>DPIHYDKITEEINKAIDDAIAAIEQSETIDPMKVPDHADKFERHVGILDFKGELAMRNIEARGLKQMKRQGDANVKGEEGIVKAHLLIGVHDDIVSMEYDLAYKLGDLHPTTHVISDIQDFVVALSLEIPDEGNITMTSFEVRQFANVVNHIGGLSILDPIFGVLSDVLTAIFQDTVRKEMTKVLAPAFKRELEKN[2x]

For decades, the house dust mite has been known as a major causative agent of various allergic diseases including asthma, atopic dermatitis (AD) and allergic rhinitis. The homologous allergen, Der f 7, isolated from D. farinae, is a 196-residue protein with 86% identity to Der p 7. Here, we report the crystal structure of Der f 7 that shows an elongated and curved molecule consisting of two anti-parallel β-sheets – one 4-stranded and the other 5-stranded – that wrap around a long C-terminal helix. In Der f 7, Leu48 and Phe50 are in close proximity to Asp159, explaining why monoclonal antibody binding to Leu48 and Phe50 can inhibit IgE binding to Asp159. Both Der f 7 and Der p 7 bind weakly to polymyxin B via a similar binding site that is formed by the N-terminal helix, the 4-stranded β-sheet and the C-terminal helix.

We purified a Der f 7 construct (Asp1 to Asn196) and determined its crystal structure by molecular replacement method. In this isoform of Der f 7, residue 130 is a Pro instead of a Ser, as reported in other Der f 7 sequences; the other residues are identical. The model of Der f 7 was refined up to a resolution of 2.0Å with R-factor of 0.224 (Rfree  = 0.28). The electron density for the N-terminal residues from Asp1 to Tyr5 and the C-terminus residue Asn196 were disordered and these residues were not included in the model. In the crystal structure of Der f 7, the 11 β-strands are arranged to form an elongated, curved anti-parallel β-sheet that wraps around the long C-terminal helix, α2; this is compared with the 10 β-strands in Der p 7. The N-terminal helix, α1, interacts closely with the 4-stranded β-sheet and the C-terminal end of the helix α2 to form a hydrophobic channel, likely for ligand binding. The ExPASy predicted isoelectric points of Der f 7 and Der p 7 as 4.90 and 4.85, respectively. Superposition of Der f 7 and Der p 7 showed that, with the exception of the N- and C-termini, the only region that is not structurally equivalent lies at the loop between β1 and β2, which harbors the largest conformational difference between these two proteins. Notably, this loop contains the linear epitope residues, Leu48 and Phe50, for the mAb HD12 that was found to inhibit IgE binding to Der f 7; these mAb epitope residues are unique to Der f 7 and found to be replaced with Ile48 and Leu50 in Der p 7. The putative IgE epitope residue of Der f 7 and Der p 7, Asp159, is located at the start of helix α2 and in proximity of the β1–β2 loop. In Der f 7, Asp159 is located closely to the β1–β2 loop with a distance of only 7.7Å between Asp159 OD1 and Phe50 CZ.>[2x]GPHMELHFNLELVETYKSNSQKARILTEDWVYRQSYCPNCGNNPLN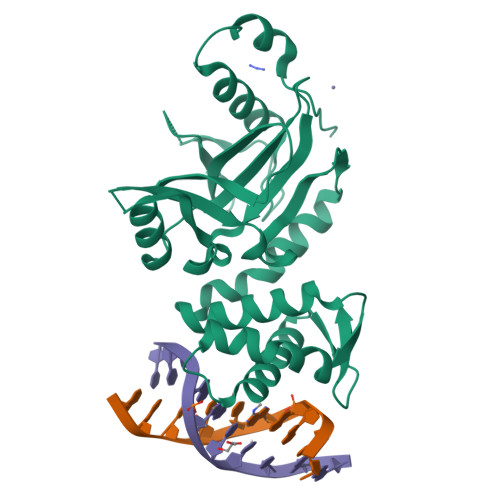HFENNRPVADFYCNHCSEEFELKSKKGNFSSTINDGAYATMMKRVQADNNPNFFFLTYTKNFEVNNFLVLPKQFVTPKSIIQRKPLAPTANRAGWIGCNIDLSQVPSKGRIFLVQDGQVRDPEKVTKEFKQGLFLRKSSLSSRGWTIEILNCIDKIEGSEFTLEDMYRFESDLKNIFVKNNHIKEKIRQQLQILRDKEIIEFKGRGKYRKL>[2x]SNAMTTDSVTQGVAHSVNGRLPELDFENRPSGAKLGIFDLPKLEVSVAPFTLAHIRVPGGVTTAEDHHEVREIWLVQSGSGILTLDGVRSRVRAGDTLYY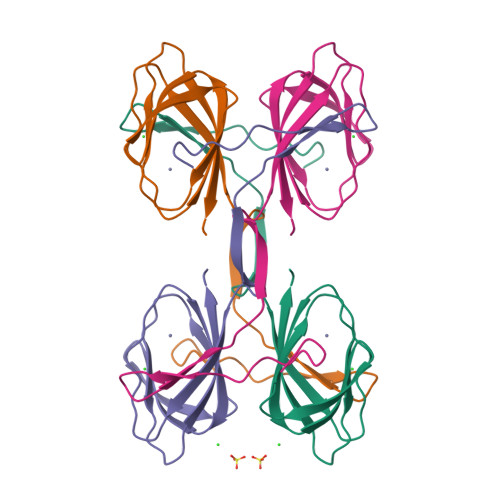ESYRRHQLHNDGDSPVEIVSIWWRP>[2x]GSSHSSANEDMPVERILEAELAVEPKTETYVEANMGLNPSSPNDPVTNICQAADKQLFTLVEWAKRIPHFSELPLDDQVILLRAGWNELLIASFSHRSIAVK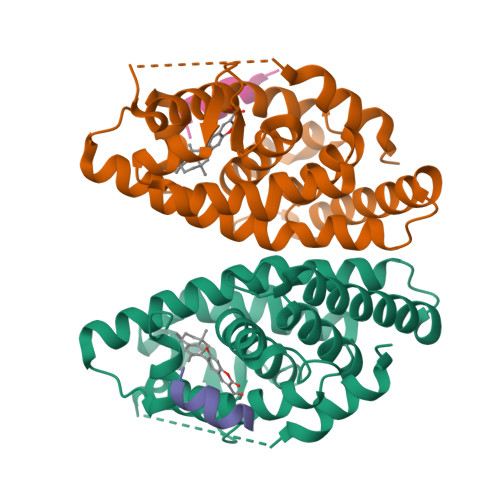DGILLATGLHVHRNSAHSAGVGAIFDRVLTELVSKMRDMQMDKTELGCLRAIVLFNPDSKGLSNPAEVEALREKVYASLEAYCKHKYPEQPGRFAKLLLRLPALRSIGLKCLEHLFFFKLIGDTPIDTFLMEMLEAPHQMT;>HKILHRLLQEGS[2x]> SNASNQTVNPQGNDQVSEASTVEITDVHGTVTVPVNPKNVVALDNRTFETLSDWGIELAAVPKPVMPADSPYVKDESVQDIGSHGEPNLEIIAAVDPELVIVGQRFARFYDDIKKLVPNAAVIDLNFDVSTEADAPGENLVNGLKDSTIALGQIFDKNKEAEQLVADFDQAIAEAKSAYNGTDTVMSVVVSGGNIGFSAPHSGRVWGPMYEIFGWTPALKIDGASSDHQGDDVSVEAIAQSNPDWIFVLDRDAAVSSMTDAVPAQDVIDKSPALQ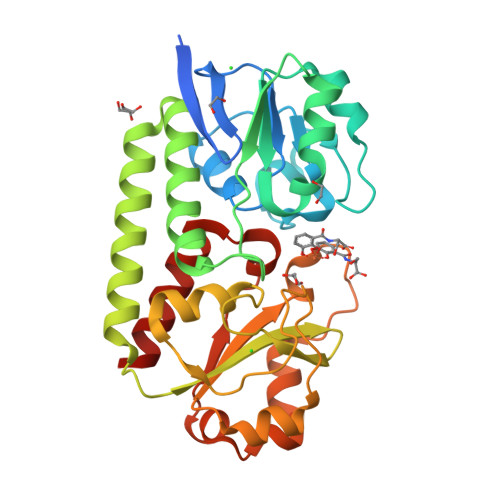KTTAVSKGQIVYAPKDTYTNESIQTYLELFEELAKALTK>MIVPVLSRQALRHASVARVALPSLTRWYASYPPHTVVKMPALSPTMTSGGIGAWQKKPGDKIEPGEVLVEIETDKAQMDFEFQEEGVLAKILKDSGEKDVAVGNPIAILVEEGTDVNAFKDFTLKDAGGETSPAVPKDEPKNESTASAPTPAPTPAPEPENTSFTGRFQTALEREPNALPAAKRLAREKGIDLRNVKGSGPGGKITEEDVKKALASAPAAGAAAAAYTDVPISGMRKTIAARLKESVTENPHFFVSTNLSVSKLLKLRQALNSSADGRYKLSVNDFLIKAMGIASKRVPTVNSSWRDGVIRQFETVDVSVAVATPNGLITPIVKGVEGKGLESISAAVKELAKKARDGKLKPEEYQGGSISISNMGMNPAVQSFTAIINPPQAAILAVGAPQKVAVPVENEDGTTGVSWDEQIIVTASFDHKVVDGAVGAEWIRELKKVIENPLELLL[60x]

The pyruvate dehydrogenase complex (PDC) catalyzes the further formation of acetyl-coenzyme A (acetyl-CoA) from pyruvate, enabling the tricarboxylic acid cycle that sustains oxidative phosphorylation. The PDC is a multienzyme complex consisting of three components: E1, E2, and E3. E2 then covalently links this acetyl group to CoA through its catalytic domain. Without exception, the PDC is organized by non-covalent recruitment of E1 and E3 to a large core built from E2 catalytic domains.

In order to characterize the fungal PDC, we purified intact complexes from N. crassa mitochondria and reconstructed its native structure from single-particle cryo-EM data. This showed a dodecahedron-shaped core with icosahedral symmetry, composed of 60 E2 core-forming domains decorated with many flexibly tethered enzymes surrounding it. While this alone did not aid the interpretation of the interior density for any such sub-symmetry, 3D classification coupled with the application of tetrahedral symmetry yielded a correctly averaged reconstruction symmetry, evidenced by a protein-like density and consistent background in the complementary interior volume. The first class has four interior, threefold symmetric densities, each immediately interior to an E2 trimer. The only observable points of contact with the E2 core are in the twofold interface bridges connecting the density-associated E2 trimer to each of its three neighbors. E2 here provides a predominantly hydrophobic pocket, composed of the C-terminal residues that form the bridge and helix 2 (H2E2). The segment of the interior density that binds to the E2 bridge pocket comprises a small (approximately seven residues) alpha-helical segment, here referred to as the binding helix (BH). The backbone and direction of the BH could be traced from our reconstructions, but the resolution did not permit assignment of its primary sequence. The cryo-EM reconstruction of the N. crassa PDC core exhibits strict icosahedral symmetry, but with an additional protein PX that forms a tetrahedral assembly interior to the core under optimal conditions. Two distinct tetrahedral configurations could be identified and refined to  ~4 Å resolution.(2,5-dihydro-1H-pyrrol-1-yl)(3-fluorophenyl)methanone | C11 H10 F N O | 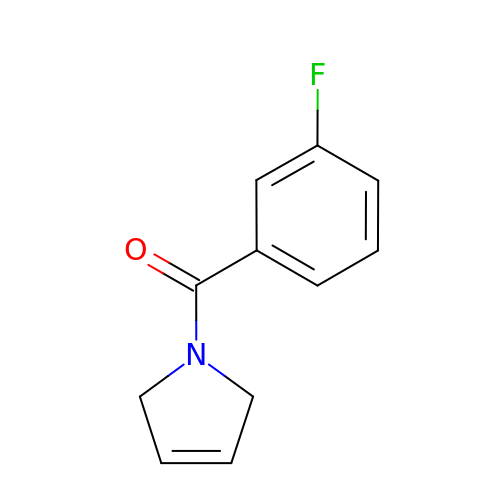IGCBBGNMEVMXTB-UHFFFAOYSA-N3'-DEOXY-CYTIDINE-5'-TRIPHOSPHATE | C9 H16 N3 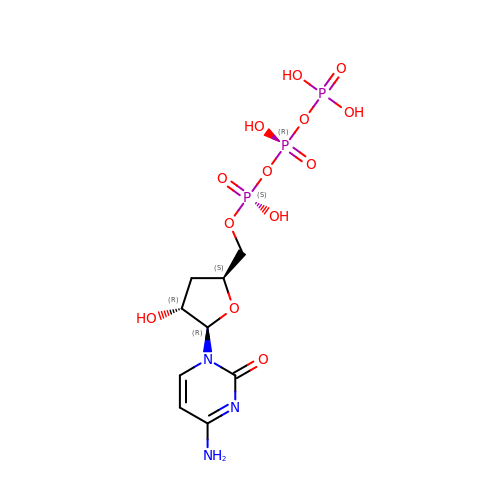O13 P3 | CHKFLBOLYREYDO-SHYZEUOFSA-N4-cyclopropyl-2-(2-hydroxyethyloxy)-N-[(1S,3R)-5-oxidanyl-2-adamantyl]-1,3-thiazole-5-carboxamide | C19 H26 N2 O4 S | 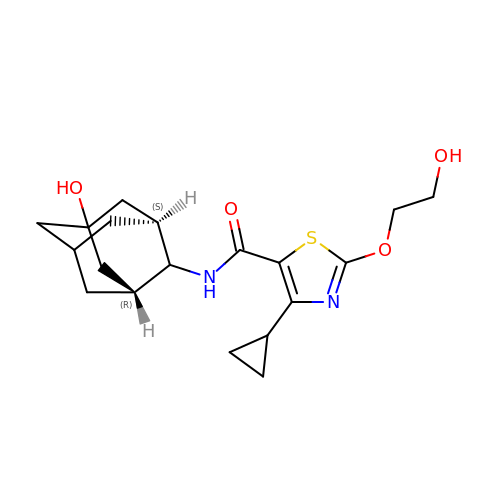NJXRHIKVLFLBME-WCUHCKLXSA-N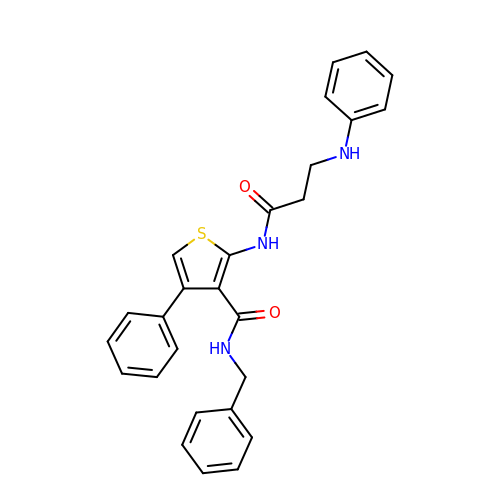N-benzyl-4-phenyl-2-[(N-phenyl-beta-alanyl)amino]thiophene-3-carboxamide | C27 H25 N3 O2 S | CDYLPAHZUJIEAN-UHFFFAOYSA-N DECANE-1-THIOL | C10 H22 S | 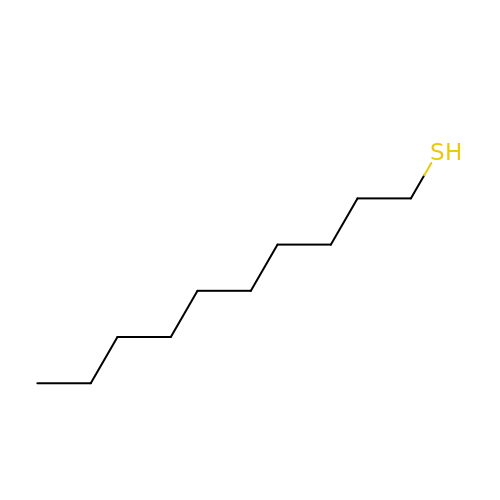VTXVGVNLYGSIAR-UHFFFAOYSA-N3-methylbut-3-enylsulfanyl(phosphonooxy)phosphinic acid | C5 H12 O6 P2 S | 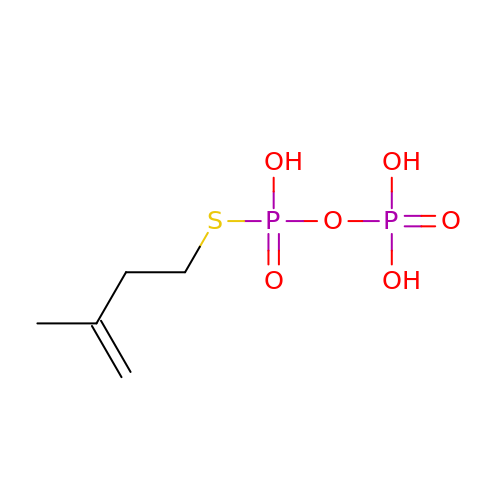YLTQZUVQWVAPNP-UHFFFAOYSA-N> MAHHHHHHMTESPASARLDRYDDAVAQFDIAKAIALLAGNPDTGINACIECCDRYTGENRVALRAISIDNTLTELTFEDLRDMSARVGNMLADAGISAGDVVAGLLPRTPELVATILGAWRIGAIYQPLFTAFGPKAIEQRFGTSGAKLVVTNLANRSKLAEVENCPRVATILAPGESLPEGDIDFRAAVAAASTECEPVMRKGSDLFMMMSTSGTAGLPKGVPVPLRALMAFGAYMRDAVGLRSDDIFWNIADPGWAYGLYYAVTGPLLLGVPTILNEGGFTAENTYDIIERLGVTSLAGSPTAFRLLIAAGPESAARVKGRLRVVSSAGEPLNPEVIRWFDACLGAPIHDHYGQTELGMVVNNHHGLEHPVRQGSAGYAMPGYRVAVLDEAGKEVGPNEPGVLAIDIDNSPLLWFTGYYKKDTPSISGGYYRTGDTVEFEPDGSISFIGRADDVITSSGYRIGPFDVESALLKHPAVNEAAVVGVPDPQRTEIVKAFVILAPGFEGTPE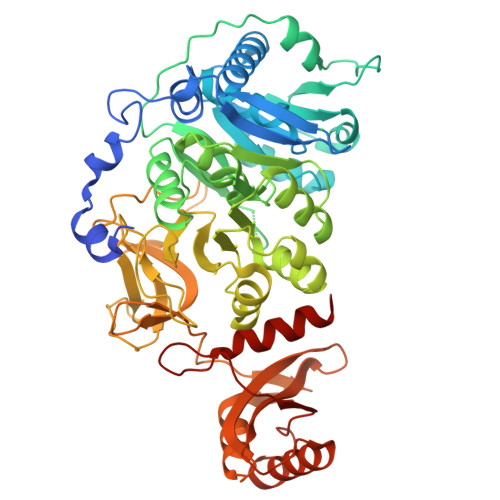LAEELALHVKKQLSAHAYPRQIDFVAELPKTPSGKIQRFLLRKAEVEKQQQQN> MGSSHHHHHHSQDPNSLEVLFQGPMAGGRDRGDLAARQLVFLLPEHLKDASKKKKKSSLLFVKLANPHSGEGATYLIDMCLQQLFEIKVFKEKHHSWFINQSVQSGGLLHFATPMDPLFLLLHYLLKAGKEGKYQPLDQVVVDDTFPDCTLLLRFPELEKSLRHVTEEKEVNSKKYYKYSSEKTLKWLEKKVNQTVVALKANNVNVGARVQSSAYFSGGQVSRDKEEDYVRYAHGLISDYIPKELSDDLSKFLKLPEPPASLTNPPSKKLKLSDEPVEAKEDYTKFNTKDLKTG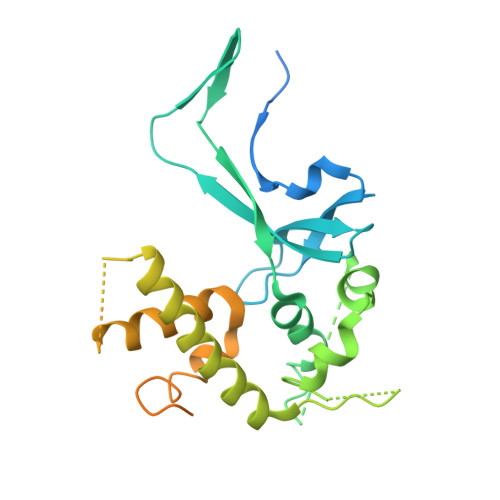KKNSKMTAAQKALAKVDKSGMKSIDAFFGAKNKKTGKI>QVEGKTQKAVCVIYPTQDYKVTGVITFTKSDDGVKVVADLNGLSPGKHGFH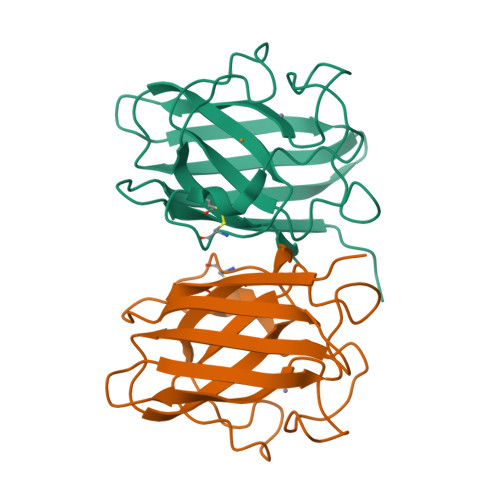IHECGDCSASDGTSAGGHFNPEEKSHGAPMDMSRHIGDLGNITADENGKAHLEYIDKMIVFEGEHSIIGRSMIVHKNEDDLKTQPTGNAGARVACGVIGIGK[4x]> MEYQHWLREAISQLQASESPRRDAEILLEHVTGRGRTFILAFGETQLTDEQCQQLDALLTRRRDGEPIAHLTGVREFWSLPLFVSPATLIPRPDTECLVEQALARLPEQPCRILDLGTGTGAIALALASERPDCEIIAVDRMPDAVSLAQRNAQ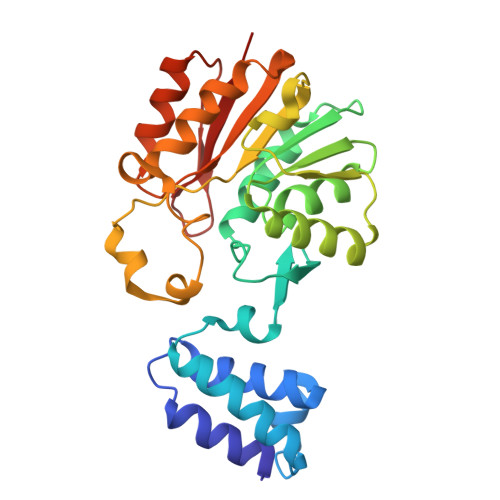HLAIKNIHILQSDWFSALAGQQFAMIVSNPPYIDEQDPHLQQGDVRFEPLTALVAADSGMADIVHIIEQSRNALVSGGFLLLEHGWQQGEAVRQAFILAGYHDVETCRDYGDNERVTLGRYY>MADHWSQAALYAEVQQHQARQMHALDEGKFEEYADTFTPDGVFRHTPGRDPAIGREAIVRELNEFHERYAEDPVQRRHMFTMLAIDELDELDDSAVQADFYTLVLTTRVDGLTVGPSCPVRDVLVRGADGRLLTASRWVE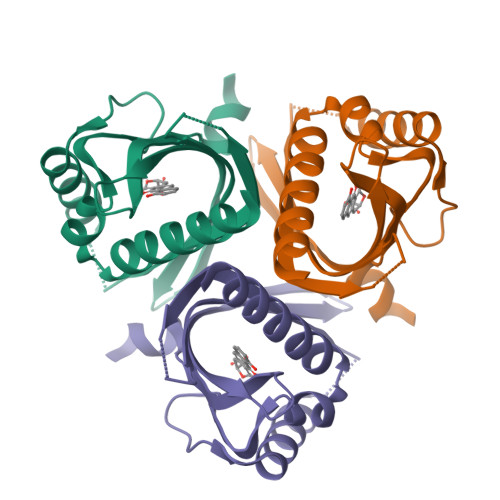HDNRTVAERTAAAR[2x]> SMGHSNRQSDVRIKFEHNGERRIIAFSRPVKYEDVEHKVTTVFGQPLDLHYMNNELSILLKNQDDLD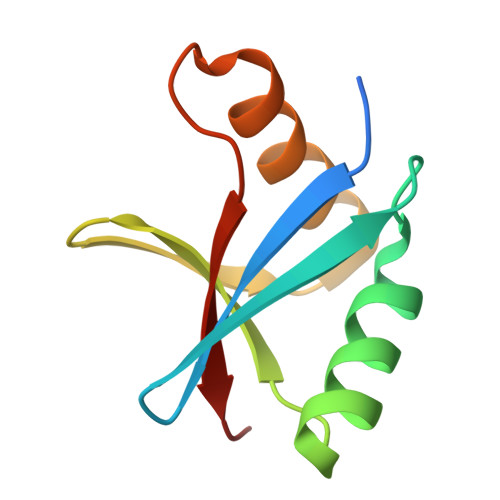KAIDILDRSSSMKSLRILLLSQD> DAFYKREMFDPAEKYKMDHRRRGIALIFNHERFFWHLTLPERRGTCADRDNLTR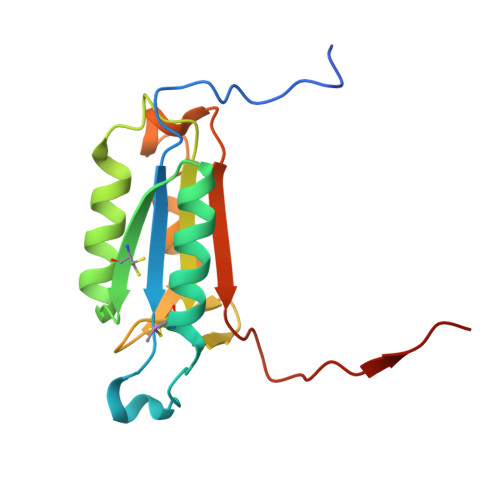RFSDLGFEVKCFNDLKAEELLLKIHEVSTVSHADADCFVCVFLSHGEGNHIYAYDAKIEIQTLTGLFKGDKCHSLVGKPKIFIIQACRGNQHDVPVIPLDVVD Maintaining the optimal nucleotide balance required for normal cell proliferation is controlled by 5′-nucleotidases amongst other processes. These enzymes catalyze the dephosphorylation of ribo- and deoxyribonucleoside monophosphates to their corresponding nucleosides, and also exhibit, in certain cases phosphotransferase activity. All structures adopt a tetrameric assembly displaying a cross-like shape, in agreement with the quaternary solution structure. Each subunit consists of four domains: an “N-Terminal Regulatory Domain” (NTRD, M1 to K59), an “OD” (D60 to T143), a HAD-like Catalytic Domain (CD, F144 to K270 and K371 to Q444) and a C2 cap domain13 (K271 to N370).

Deletion of the 30 N-terminal residues (PfISN1-∆N30) leads to a threefold increased activity at both pH 8 and pH 5. This deletion mutant at pH 8 shows twofold increase in kcat(app) with a similar fold lowering of Km(app) value. The structure of PfISN1D172N-∆N30 co-crystallized with IMP (PfISN1D172N-∆N30-IMP) is similar to the PfISN1D172N-IMP structure (RMSD = 0.46 Å), confirming that only residues 30–59 are mandatory for stabilizing SegmentD394-F407 in conformation. As concerns the IMP-binding stoichiometry, we observed that in the PfISN1D172N-IMP structure, each subunit binds one IMP-Mg2+, a feature also observed in the PfISN1D172N-ΔN30-IMP structure. We also showed that whereas residues 30–59 are directly involved in the catalytic mechanism, residues 1–29 rather contribute to a global stabilization of the structure during conformational changes associated with catalytic function. The crystal structures confirm that the IMP-Mg2+ substrate is mainly coordinated by conserved residues from the four HAD motifs, and by W365, which is situated on β-strand I. The base moiety of the nucleotide is stabilized by a π-stacking interaction with W365 and by three hydrogen bonds with A205 (Motif II), S207 and D367. Hydroxyl groups 2′ and 3′ of the sugar moiety form hydrogen bonds with D363 and D178, respectively, whereas the phosphate moiety of the nucleotide forms hydrogen bonds with D170 (Motif I), T204 and A205 (Motif II), K371 (Motif III), and N401 (Motif IV). Mg2+ is coordinated by the phosphate moiety, side chains of D170 (Motif I), D394 and Q395 (Motif IV), and the main chain carbonyl of D/N172.

>SDRNVMNSDMKKNIVQWNSRYSYNQLKNKDSLIMFLVEIFRSLFVSNCIDKNIDNVLLSIEEMFIDHYYNPQHSRLKYLIDDVGIFFTKLPITKAFHTYNKKYRITKRLYAPPTFNEVRHILNLAQILSLEEGLDLLTFDANETLYPDGHDFNDEVLASYISCLLKKMNIAIVTAASYNNDAEKYQKRLENLLKYFSKHNIKDGSYKNFYVMGGESNYLFKCNEEATLYSVPENEWRHYKKFVDYDTVQEILNISEKCLEKVIKDFGLCAQIQRKEKSIGLVPNKIPSLNIKNEQKNYMIKYEVLEEAVIRIKKEIIKNKITAPYCAFNGGQDLWVDVGNKAEGLLILQKLLKIQKKKCCHIGDQFLHSGNDFPTRFCSLTLWVSNPQETKACLKSIMHLNIKSFIPEVLYENQ[8x]> ALTYRGADISSLLLLEDEGYSYKNLNGQTQALETILADAGINSIRQRVWVNPSDGSYDLDYNLELAKRVKAAGMSLYLDLHLSDTWADPSDQTTPSGWSTTDLGTLKWQLYNYTLEVCNTFAENDIDIEIISIGNEIRAGLLWPLGETSSYSNIGA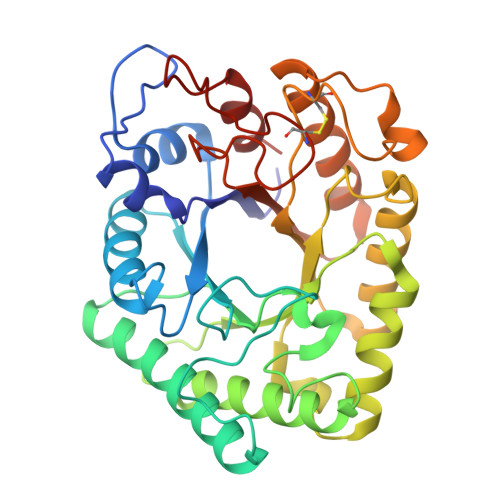LLHSGAWGVKDSNLATTPKIMIHLDDGWSWDQQNYFYETVLATGELLSTDFDYFGVSYYPFYSASATLASLKTSLANLQSTYDKPVVVVETNWPVSCPNPAYAFPSDLSSIPFSVAGQQEFLEKLAAVVEATTDGLGVYYWEPAWIGNAGLGSSCADNLMVDYTTDEVYESIETLGEL> MARPIDVSQLIAGINKKKGLDENTSGKISKPRFLNKQERSKQERLKENEESLTPTQSDSAKVEIKKVNSRDDSFFNETNDKKRNPSKQNGSKFHFSWNESEDTLSGYDPIVSTRAIDLLWKGKTPKNAAESSYMGKHWTEKSLHEMNERDWRILKEDYAIVTKGGTVENPLRNWEELNIIPRDLLRVIIQELRFPSPTPIQRITIPNVCNMKQYRDFLGVASTGSGKTLAFVIPILIKMSRSPPRPPSLKIIDGPKALILAPTRELVQQIQKETQKVTKIWSKESNYDCKVISIVGGHSLEEISFSLSEGCDILVATPGRLIDSLENHLLVMKQVETLVLDEADKMIDLGFEDQVTNILTKVDINADSAVNRQTLMFTATMTPVIEKIAAGYMQKPVYATIGVETGSEPLIQQVVEYADNDEDKFKKLKPIVAKYDPPIIIFINYKQTADWLAEKFQKETNMKVTILHGSKSQEQREHSLQLFRTNKVQIMIATNVAARGLDIPNVSLVVNFQISKKMDDYIHRIGRTGRAANEGTAVSFVSAAEDESLIRELYKYVRKHDPLNSNIFSEAV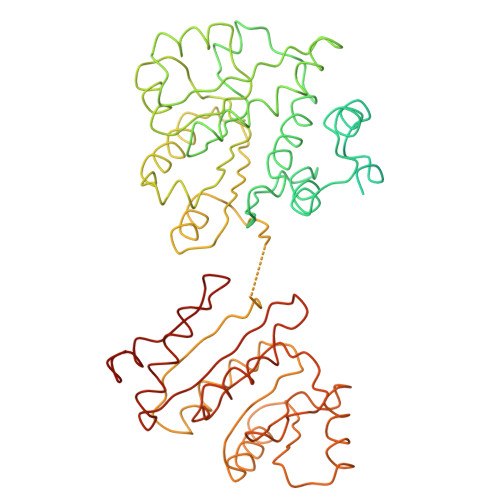KNKYNVGKQLSNEIIY>[5x]SLINTKIKPFKNQAFKNGEFIEVTEKDTEGRWSVFFFYPADFTFVCPTELGDVADHYEELQKLG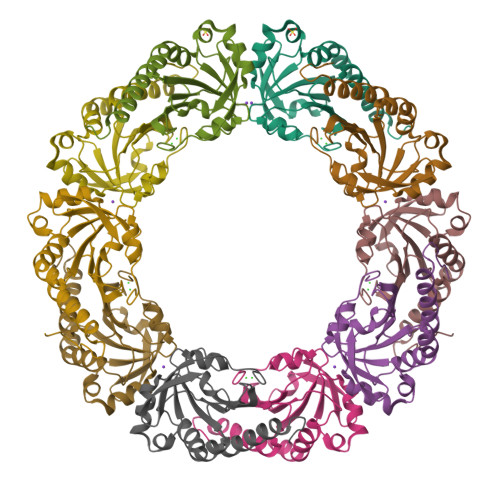VDVYSVSTDTHFTHKAWHSSSETIAKIKYAMIGDPTGALTRNFDNMREDEGLADRATFVVDPQGIIQAIEVTAEGIGRDASDLLRKIKAAQYVAAHPGEVCPAKFKEGEATLAPSLDLVGKI[2-[3-[(4-azanyl-2-methyl-pyrimidin-5-yl)methyl]-4-methyl-1,3-thiazol-5-yl]ethoxy-oxidanyl-phosphoryl]methylphosphonic 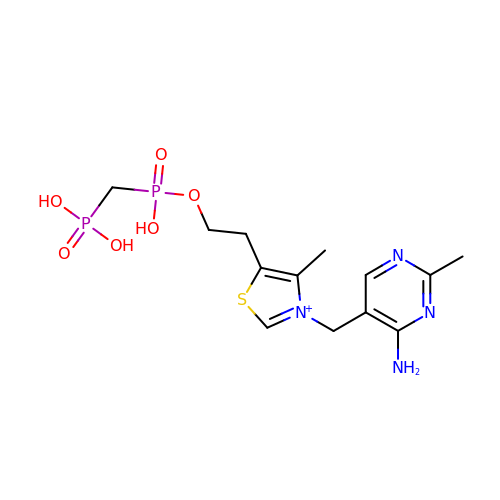acid | C13 H21 N4 O6 P2 S | NSFCGDWNWBEOER-UHFFFAOYSA-O>CGAAUXCG[1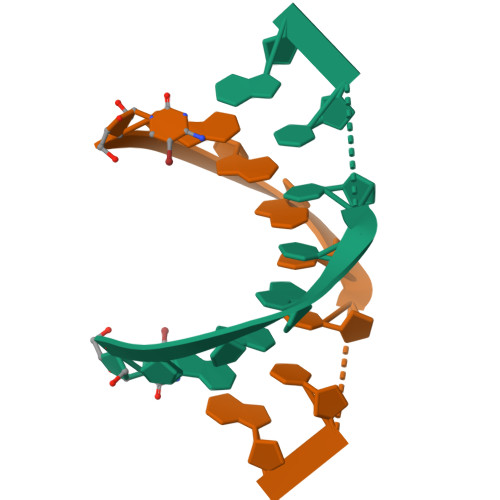4x]> SMT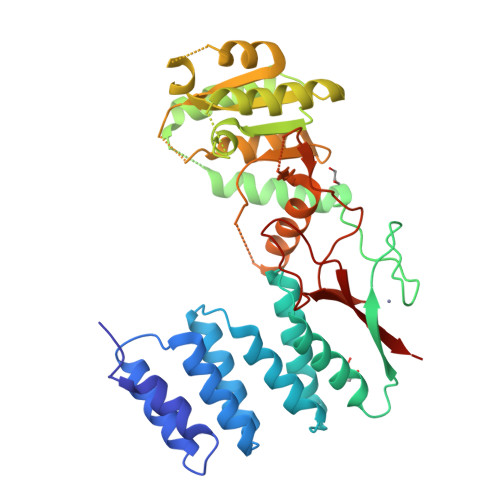LEPRGYSLLIRGLIHSDRWREALLLLEDIKKVITPSKKNYNDCIQGALLHQDVNTAWNLYQELLGHDIVPMLETLKAFFDFGKDIKDDNYSNKLLDILSYLRNNQLYPGESFAHSIKTWFESVPGKQWKGQFTTVRKSGQCSGCGKTIESIQLSPEEYECLKGKIMRDVIDGGDQYRKTTPQELKRFENFIKSRPPFDVVIDGLNVAKMFPKVRESQLLLNVVSQLAKRNLRLLVLGRKHMLRRSSQWSRDEMEEVQKQASCFFADDISEDDPFLLYATLHSGNHCRFITRDLMRDHKACLPDAKTQRLFFKWQQGHQLAIVNRFPGSKLTFQRILSYDTVVQTTGDSWHIPYDEDLVERCSCEVPTKWLCLHQKT>GSELRSIAFSRAVFAEFLATLLFVFFGLGSALNWPQALPSVLQIAMAFGLGIGTLVQALGHISGAHINPAVTVACLVGCHVSVLRAAFYVAAQLLGAVAGAALLHEITPADIRGDLAVNALSNSTTAGQAVTVELFLTLQLVLCIFASTDERRGENPGTPALSIGFSVALGHLLGIHYTGCSMNPARSLAPAVVTGKFDDHWVFWIGPLVGAILGSLLYNYVLFPPAKSLSERLAVLKGLEP[4x]

Here, a new method of on-chip crystallization is reported which allows the efficient and reproducible growth of large numbers of protein crystals directly on micro-patterned silicon chips for in-situ serial crystallography experiments. Crystals are grown by sitting-drop vapor diffusion and previously established crystallization conditions can be directly applied. As a consequence, ‘naked’ crystals are obtained on the chip, resulting in very low background scattering levels and making the crystals highly accessible for external manipulation such as the application of ligand solutions. Serial diffraction experiments carried out at cryogenic temperatures at a synchrotron and at room temperature at an X-ray free-electron laser yielded high-quality X-ray structures of the human membrane protein aquaporin 2 and two new ligand-bound structures of thermolysin and the human kinase DRAK2.

We collected serial diffraction data for on-chip crystallized human aquaporin 2 (hAQP2) at room temperature at LCLS using the fast-scanning Roadrunner II goniometer. From two Roadrunner II chips we obtained 3377 hits from 137 476 collected frames (a 2.5% hit rate), leading to 2723 indexed patterns (an 80.6% indexing rate). The rod-shaped hAQP2 crystals showed a strong preference for two distinct orientations rotated along their long fourfold symmetry axis when lying on the flat silicon-chip surface. The corresponding diffraction patterns collected with a beam perpendicular to the chip plane hence show a strong bias and Bragg peaks only cover a very narrow region of reciprocal space. In order to obtain a complete data set, we tilted the chip by 25° during SX data collection. Each monomer contains a water channel surrounded by six transmembrane helices and two half-helices forming a pseudo-transmembrane helix. Despite the limited resolution of the data, clear density for a water molecule is observed in the middle of the water-conducting pore of one of the hAQP2 monomers, close to the conserved NPA region. Therefore, the weaker diffraction properties of the crystals used in this work are most likely to be owing to their significantly smaller size compared with the crystals used for previous structural determination and do not originate from our on-chip crystallization method. The hit rates of 2.5% as observed for hAQP2 on the Roadrunner II chips were low for a fixed-target experiment and can probably be attributed to the low protein concentration that was used.>[2x]ETGTVPAINYLGAGYDHVRGNPVGDPSSMGDPGIRPPVLRFTYAQNEDGVSNDLTVLQPLGGYVRQYVACRQSETISELSNLSDYQNELSVDASLQGGDPIGLNSFSASTGYRDFAKEVSKKDTRTYMLKNYCMRYEAGVAQSNHFKWNVTLAFAAGVSQLPDVFDAHNPECACSAEQWRQDQNAEACTKTNVPIWISFIEQFGTHFLVRLFAGGKMTYQVTAKRSEVEKMRNMGIDVKTQLKMQLGGVSGGAGQGTSSKKQQSSSEYQMNVQKETLVIGGRPPGQVSDPAALAAWADTVEELPMPVKFEVQPLYHLLPVEKQEAFKQAVTFYSKAVGLTPQDLSALGTKHHHHHH

Toxoplasma and Plasmodium are the parasitic agents of toxoplasmosis and malaria, respectively, and use perforin-like proteins (PLPs) to invade host organisms and complete their life cycles. Escape from the PV, and therefore from the infected cell, for subsequent rounds of infection has been shown to be dependent on the perforin-like protein TgPLP1 (T. gondii PLP). We report structures of the membrane attack complex/perforin (MACPF) and Apicomplexan PLP C-terminal β-pleated sheet (APCβ) domains of TgPLP1. The MACPF domain forms hexameric assemblies, with ring and helix geometries, and the APCβ domain has a novel β-prism fold joined to the MACPF domain by a short linker.

Molecular replacement in the same way was also used to solve the structure of an intact monomeric form of the MACPF domain at 3.11 Å in space group C2. In addition to the core-bent β sheet, we were able to resolve the whole of the TMH1 region (helices α1 and α2) and two parts of the TMH2 region (helices α7 and α8), although the TMH2 region was partly disordered and thus not visible in the crystal structure. Whereas TMH1 is packed into a pocket, TMH2 is more exposed to solvent, explaining its mobility. In addition to a further set of helices that cap the top of the core β sheet, we noted two helical inserts (α4 and α5) not present in other MACPF domains to have had their structures resolved and that α9 is angled out from the core of the domain. Together, these features cause the TgPLP1 MACPF domain to be somewhat bulkier than other perforin-like proteins, which partly explains its capacity to form much smaller oligomers than other family members (see below).>[3x]MNDHEVDVLVVGAGLGGLSTAMFLARQGVRVLVVERRPGLSPYPRAAGQNPRTMELLRIG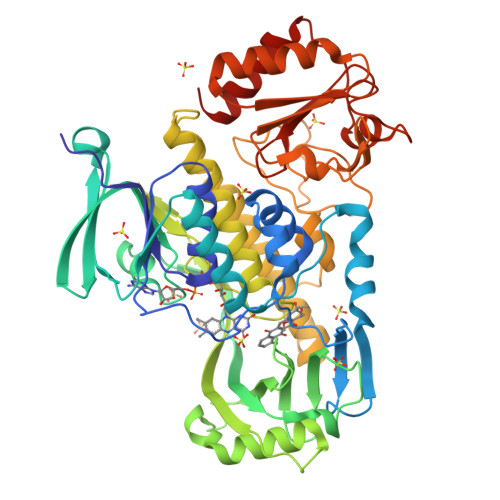GVADEVVRADDIRGTQGDFVIRLAESVRGEILRTVSESFDDMVAATEPCTPAGWAMLSQDKLEPILLAQARKHGGAIRFGTRLLSFRQHDDDAGAGVTARLAGPDGEYDLRAGYLVGADGNRSLVRESLGIGRYGHGTLTHMVGVIFDADLSGIMEPGTTGWYYLHHPEFKGTFGPTDRPDRHTLFVEYDPDEGERPEDFTPQRCVELIGLALDAPEVKPELVDIQGWEMAARIAERWREGRVFLAGDAAKVTPPTGGMSGNAAVADGFDLAWKLAAVLQGQAGAGLLDTYEDERKVAAELVVAEALAIYAQRMAPHMAEVWDKSVGYPETLLGFRYRSSAVLATDDDPARVENPLTPSGRPGFRGPHVLVSRHGERLSTVDLFGDGWTLLAGELGADWVAAAEAVSAELGVPVRAYRVGAGLTDPESAVSERYGIGKAGASLVRPDGIVAWRTDEAAADAAQTLEGVLRRVLDR> XXXXXXXXXXXXXXXXXXXXXXXXXXXXXXQQLLDIISEFILLGLNPEPVCVVLKKSPQLLKLPIMQMRKRSSYLQKLGLGEGKLKRVLYCCPEIFTMRQQDINDTVRLLKEKCLFTVQQVTKILHSCPSVLREDLGQLEYKFQYAYFRMGIKHPDIVKSEYLQYSLTKIKQRHIYLERLGRYQTPDKKGQTQIPNPLLKDILRVSEAEFLARTACTSVEE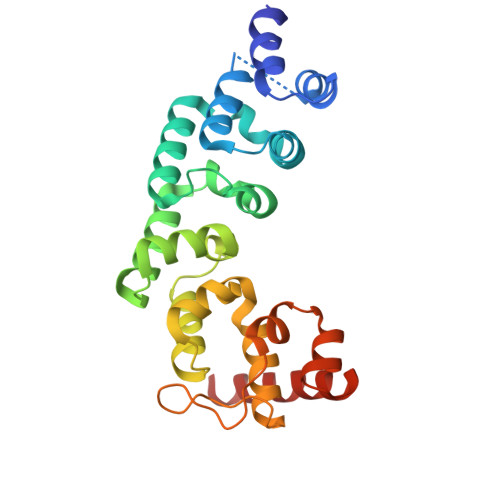FQVFKKLLAREEEESESS>MINMODELKKLFLVFWWHMHQPLYREPYTGEYLLPWTFFHAVKDYYDMPAYLKDFEIKLNFNLTPVLIDQIQEYAQGKAKDVFLEAIRKDPDDLEKEEVEKLIEFTKLNYEKPIYRFERIRELMNKEKLNREELLDLQTLNLLAWCGRTLRKDLKDLLNKGRNYTQEEKEYVLNKYFEIIKKTLSIYREIKEEGKGSVSTSPYYHPLIPILLNPNCVYETTPNVKIPDFAVSFREDASKHVELAKEKYFEIFGEHPVYMWPPEASVSNEALELYYEKGINMLATDEVILKNSVERASPYLRYYFRELISVFFRDKTLSDLIGFSYHAWNAEDAVRDFIGRLKKIHESVDFQPVVFVVLDGENCWEYYEENGIPFLEKLYSTLEKEEWIETLTLEEAMRKEDVKTEVIESVKAGTWFDGNFLKWIGNKEKNEYWKILIEAKKKAKNDYILVAEGSDWFWWQGEEKAPFVEVFDKLFRSFVRRAQE[3x];> MKKLFLVFWWHMHQPLYREPYTGEYLLPWTFFHAVKDYYDMPAYLKDFEIKLNFNLTPVLIDQIQEYAQGKAKDVFLEAIRKDPDDLEKEEVEKLIEFTKLNYEKPIYRFERIRELMNKEKLNREELLDLQTLNLLAWCG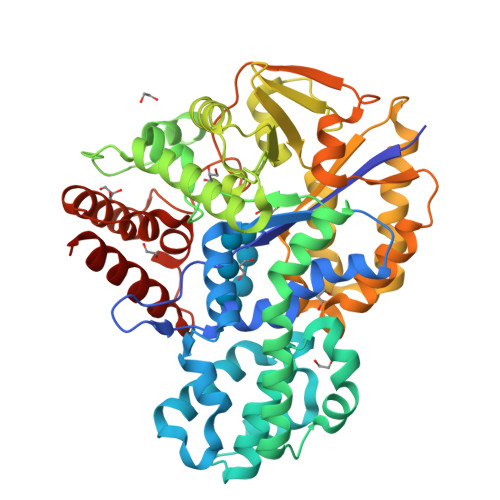RTLRKDLKDLLNKGRNYTQEEKEYVLNKYFEIIKKTLSIYREIKEEGKGSVSTSPYYHPLIPILLNPNCVYETTPNVKIPDFAVSFREDASKHVELAKEKYFEIFGEHPVYMWPPEASVSNEALELYYEKGINMLATDEVILKNSVERASPYLRYYFRELISVFFRDKTLSDLIGFSYHAWNAEDAVRDFIGRLKKIHESVDFQPVVFVVLDGENCWEYYEENGIPFLEKLYSTLEKEEWIETLTLEEAMRKEDVKTEVIESVKAGTWFDGNFLKWIGNKEKNEYWKILIEAKKKAKNDYILVAEGSDWFWWQGEEKAPFVEVFDKLFRSFVRRAQE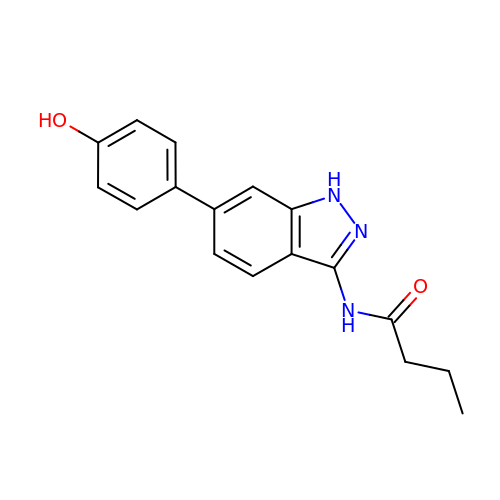N-[6-(4-hydroxyphenyl)-1H-indazol-3-yl]butanamide | C17 H17 N3 O2 | VCIZMGNKKFEEHA-UHFFFAOYSA-N>[3x]DTDGLWAALTEAAASVEKLLATLPEHGARSSAERAEIAAAHDAARALRVRFLDTHADAVYDRLTDHRRVHLRLAELVEAAATAFPGLVPTQQQLAVERSLPQAAKEGHEIDQGIFLRAVLRSPLAGPHLLDAMLRPTPRALELLPEFVRTGEVEMEAVHLERRDGVARLTM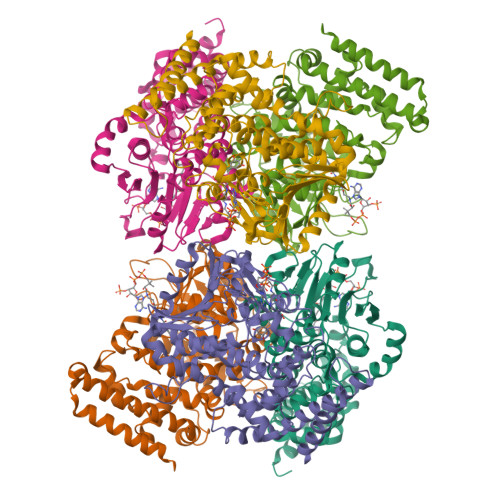CRDDRLNAEDGQQVDDMETAVDLALLDPGVRVGLLRGGVMSHPRYRGKRVFSAGINLKYLSQGGISLVDFLMRKELGYIHKLVRGVLTNDDRPGWWHSPRIEKPWVAAVDGFAIGGGAQLLLVFDRVLASSDAYFSLPAAKEGIIPGAANLRLGRFAGPRVSRQVILEGRRIWAKEPEARLLVDEVVEPDELDAAIERSLTRLDGDAVLANRRMLNLADESPDGFRAYMAEFALMQALRLYGHDVI N,N'-TETRAMETHYL-ROSAMINE | C23 H23 N2 O | 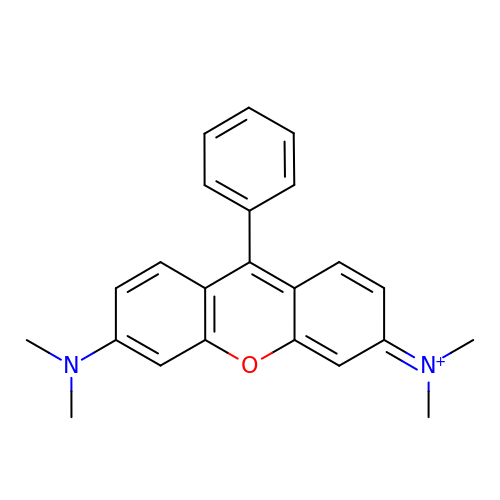NGSXFKKYKWBNPO-UHFFFAOYSA-N>[7x]VEYKNTICPPRQDYRYWYFVAELTIGVNYDINSTIIGECHMSESYIDRNANIVLTGYGLKINMTIMDTDQRFVAAAEGVGKDNKLSVLLFTTQRLDKVHHNISVTITCMEMNCGTTKYNSDLPESIHKSSSCDITINGSCVTCVNLETDPTKINPHYLHPKNKYLYHN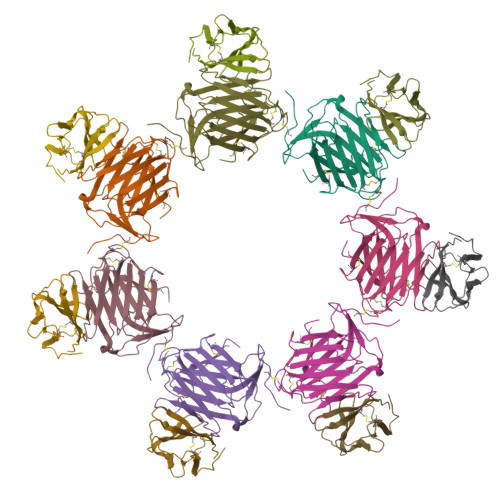SEYSMRGSYGVTFIDELNQCLLDIKELSYDICYRE;>LKIQAYFNETADLPCQFANSQNQSLSELVVFWQDQENLVLNEVYLGKEKFDSVHSKYMGRTSFDSDSWTLRLHNLQIKDKGLYQCIIHHKKPTGMIRIHQMNSELSVLANFSQPEIVPISNITENVYINLTCSSIHGYPEPKKMSVLLRTKNSTIEYDGVMQKSQDNVTELYDVSISLSVSFPDVTSNMTIFCILETDKTRLLSSPFSIELED[7x]NICOTINIC ACID ADENINE DINUCLEOTIDE | C21 H27 N6 O15 P2 | 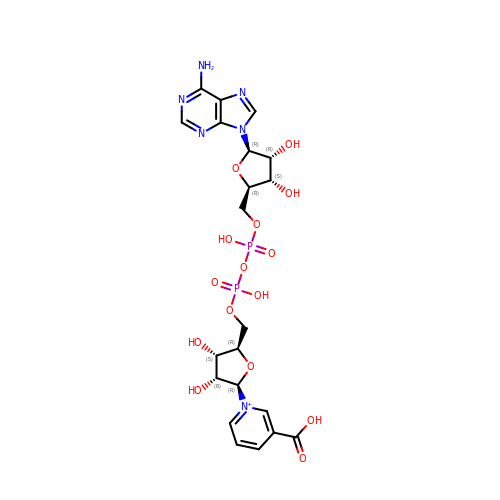SENPVEZBRZQVST-HISDBWNOSA-O N-[5-(4-methylpiperazine-1-carbonyl)[1,1'-biphenyl]-2-yl]-4-oxo-3,4-dihydrothieno[3,2-d]pyrimidine-7-carboxamide 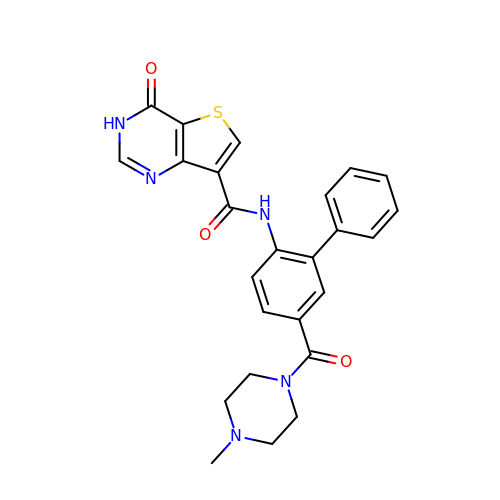| C25 H23 N5 O3 S | USMAPSJMQVFIAW-UHFFFAOYSA-N> MADKRKLQGEIDRCLKKVSEGVEQFEDIWQKLHNAANANQKEKYEADLKKEIKKLQRLRDQIKTWVASNEIKDKRQLIDNRKLIETQMERFKVVERETKTKAYSKEGLGLAQKVDPAQKEKEEVGQWLTNTIDTLNMQVDQFESEVESLSVQTRKKKGDKDKQDRIEGLKRHIEKHRYHVRMLETILRMLDNDSILVDAIRKIKDDVEYYVDSSQDPDFEENEFLYDDLDLEDIPQALVATSPPSHSHMEDEIFNQSSSTPTSTTSSSPIPPSPANCTTENSEDDKKRGRSTDSEVSQSPAKNGSKPVHSNQHPQSPAVPPTYPSGPPPAASALSTTPGNNGVPAPAAPPSALGPKASPAPSHNSGTPAPYAQAVAPPAPSGPSTTQPRPPSVQPSGGGGGGSGGGGSSSSSNSSAGGGAGKQNGATSYSSVVADSPAEVALSSSGGNNASSQALGPPSGPHNPPPSTSKEPSAAAPTGAGGVAPGSGNNSG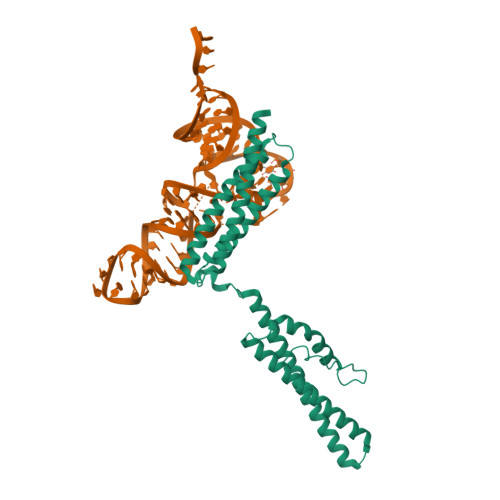GPSLLVPLPVNPPSSPTPSFSDAKAAGALLNGPPQFSTAPEIKAPEPLSSLKSMAERAAISSGIEDPVPTLHLTERDIILSSTSAPPASAQPPLQLSEVNIPLSLGVCPLGPVPLPR>GPKQIPKKPCNEKNLKEAVYDICCNGLSNNAAIIMYFTRSKKVAQIIKIMQKELMIRPNITVSEAFKMNHAPPKYYDKDEIKRFIQLQKQGPQELWDKFENNTTHDLFTRHSDVKTMIIYAATPIDFVGAVKTCNKYAKDNPKEIVLRVCSIIDGDN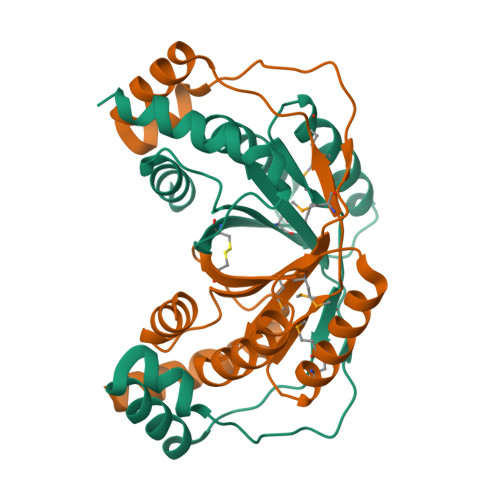PISIYNPISKEFKSKFSTLSKC[4x]5-chloro-N-[(3R)-1-(2-{[2-fluoro-4-(2-oxopyridin-1(2H)-yl)phenyl]amino}-2-oxoethyl)pyrrolidin-3-yl]thiophene-2-carboxamide 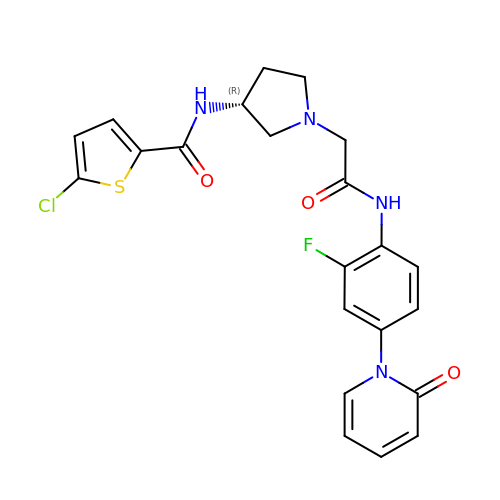| C22 H20 Cl F N4 O3 S | IYGIXVNAMZPBDK-CQSZACIVSA-N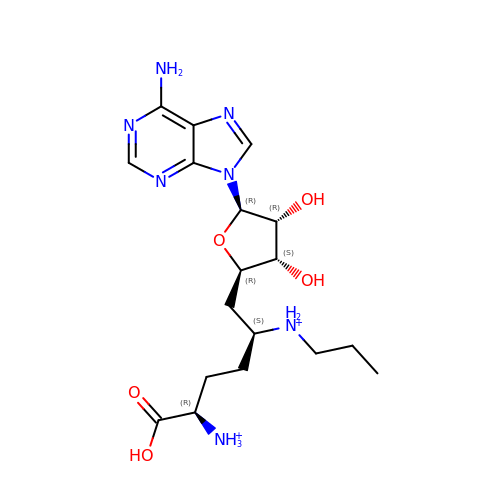[(2~{S},5~{R})-1-[(2~{R},3~{S},4~{R},5~{R})-5-(6-aminopurin-9-yl)-3,4-bis(oxidanyl)oxolan-2-yl]-5-azaniumyl-6-oxidanyl-6-oxidanylidene-hexan-2-yl]-propyl-azanium | C18 H31 N7 O5 | ZDIZXAAADLAUDS-BRZDOZMNSA-P> SNAMKIVKRALTFEDVLLRPGYSEVLPKEVKIHTKLTKNITLNMPLISAAMDTVTEHRAAIMMARLGGLGVIHKNMDIASQVREVKRVKKSESGGIKDLKKRKEYPDANKDNFGRLRVGAAIGVGQMDRVDALVEAGVDVVVLDSAHGHSKGIIDTVKAIKAKYPNLDLIAGNIATAAAAKALCEAGVDAVKVG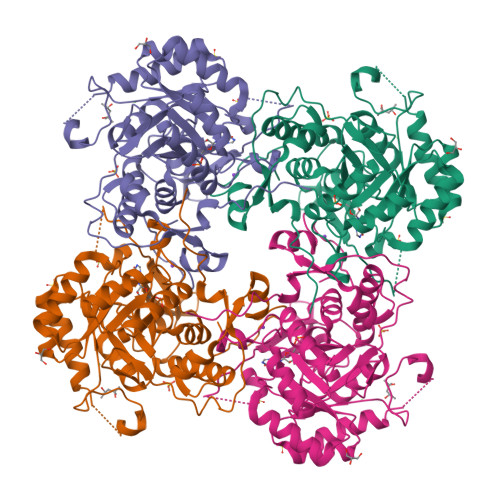IGPGSICTTRIVSGVGVPQISAIDECVEEANKFGVPVIADGGIKYSGDIAKALAVGASSVMIGSLLAGTDESPGELFTYQGRQYKSYRGMGSLGAMQKGSSDRYFQQGTAQDKLVPEGIEGRVPYVGSIRSVVHQLLGGLRSSMGYVGAKDIEDFQKRAEFVEITTAGLKESHVHDVTITHEAPNYKVNHQ> ETLP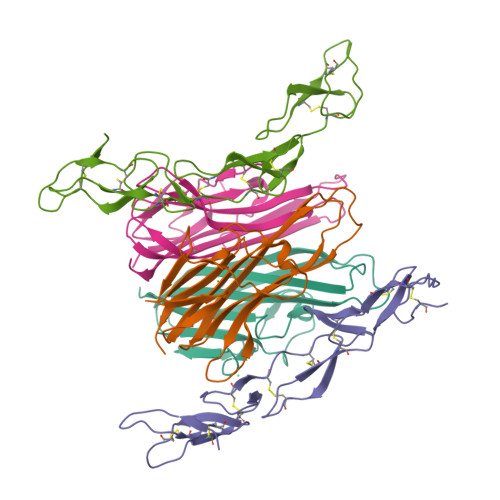PKYLHYDPETGHQLLCDKCAPGTYLKQHCTVRRKTLCVPCPDHSYTDSWHTSDECVYCSPVCKELQSVKQECNRTHNRVCECEEGRYLEIEFCLKHRSCPPGSGVVQAGTPERNTVCKKCPDGFFSGETSSKAPCIKHTNCSTFGLLLIQKGNATHDNVCSGNREATQKCGIASSVLPR;> QPFAHLTINAASIPSGSHKVTLSSWYHDRGWAKISNMTLSNGKLRVNQDGFYYLYANICFRHHETSGSVPTDYLQLMVYVVKTSIKIPSSHNLMKGGSTKNWSGNSEFHFYSINVGGFFKLRAGEEISIQVSNPSLLDPDQDATYFGAFKVQDID>[3x]ADPDMS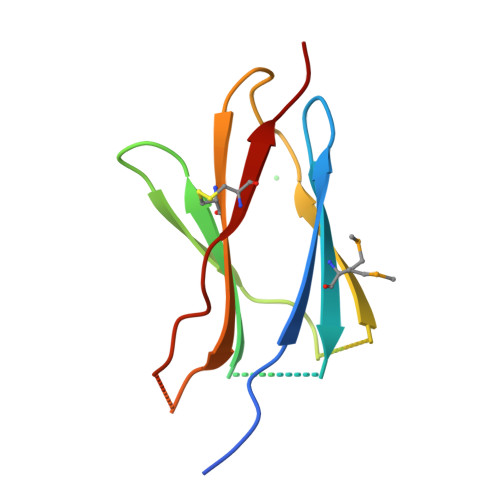FEPPEFEIVGFTNHINVMVKFPSIVEEELQFDLSLVIEEQSEGIVKKHKPEIKGNMSGNFTYIIDKLIPNTNYCVSVYLEHSDEQAVIKSPLKCTLLPP> TSNVITQD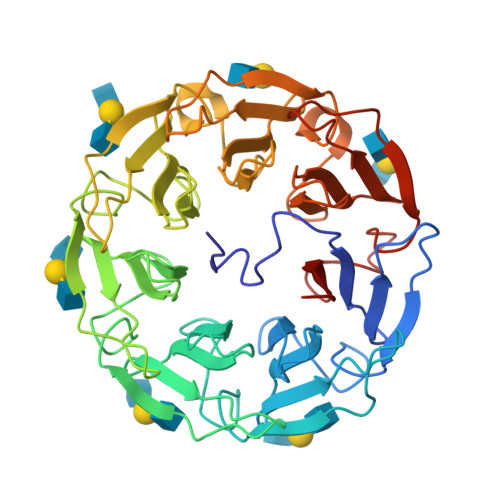LPIPVASRGFADIVGFGLDGVVIGRNAVNLQPFLAVKNFAQNAGGWLTTKHVRLIADTTGTGKGDIVGFGNAGVYVSVNNGKNTFADPPKMVIANFGYDAGGWRVEKHLRYLADIRKTGRADIIGFGEKGVLVSRNNGGLNFGPATLVLKDFGYDAGGWRLDRHLRFLADVTGNGHLDIVGFGDKHVFISRNNGDGTFAPAKSVIDNFCIDAGGWKIGDHPRFVADLTGDGTADIIGCGKAGCWVALNNGGGVFGQVKLVINDFGTDKGWQAAKHPRFIADLTGNGRGDVVGFGNAGVYVALNNGDGTFQSAKLVLKDFGVQQGWTVSKHRRFVVDLTGDGCADIIGFGEKETLVSYNDGKGNFGPVKALTNDFSFSGGKWAPETTVCWMANLDSSRH> GPGLKQKIVIKVAMEGNNCRSKAMALVASTGGVDSVALVGDLRDKIEVVGYGIDPIKLISALRKKVGDAELLQ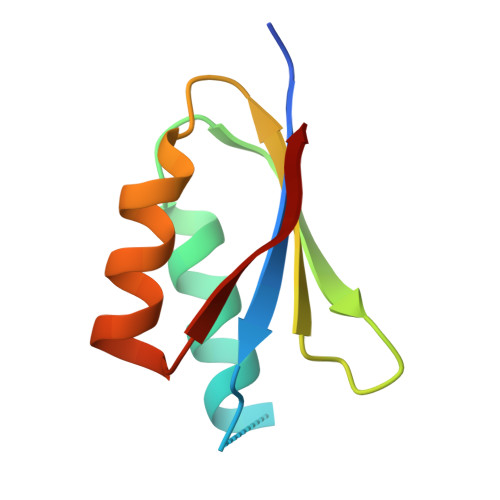VS>[2x]MKKKIIIA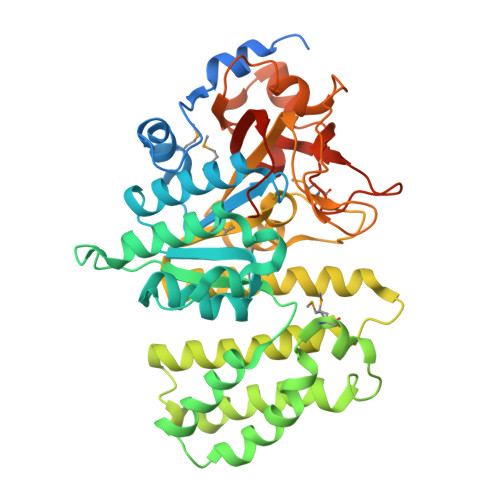IVASAITMTHFVGNTYADSKTEVSVTAPYNTNQIAKWLEAHAKPLKTTNPTASLNDLKPLKNMVGSASIVGLGEATHGAHEVFTMKHRIVKYLVSEKGFTNLVLEEGWDRALELDRYVLTGKGNPSQHLTPVFKTKEMLDLLDWIRQYNANPKHKSKVRVIGMDIQSVNENVYNNIIEYIKANNSKLLPRVEEKIKGLIPVTKDMNTFESLTKEEKEKYVLDAKTISALLEENKSYLNGKSKEFAWIKQNARIIEQFTTMLATPPDKPADFYLKHDIAMYENAKWTEEHLGKTIVWGHNGHVSKTNMLSFIYPKVAGQHLAEYYGKRYVSIGTSVYEGQYNVKNSDGEFGPYGTLKSDDPNSYNYIFGQVKKDQFFIDLRKANGVTKTWLNEQHPIFAGITTEGPDIPKTVDISLGKAFDILVQIQKVSPSQVHQLEHHHHHH> AGRLEEALELFEEMKEKGIVPDVVTYNTLISGLGKAGRLEEALELFEEMKEKGIVPDVVTYTTLISGLGKAGRLEEALELFEEMKEKGIVPNVVTYTTLISGLGKAGRLEEALELFEEMKEKGIVPDVVTYTTLISGLGKAGRLEEALELFEEMKEKGIVPDVVTYTTLISGLGKAGRLEEALELFEEMKEKGIVPDVVTYNTLISGLGKAGRLEEALELFEEMKEKGIVPDVVTYNTLISGLGKAGRLEEALELFEEMKEKGIVPDVVTYTTLISGLGKAGRLEEALELFEEMKEKGIVPNVVTYTTLISGLGKAGRLEEALELFEEMKEKGIVPDVVTYTTLISGLGK

PPR proteins are RNA-binding proteins found predominantly in mitochondria and chloroplasts. PPRs stack on each other to form an extended solenoid structure that can recognise RNA in a sequence-specific manner based on the identities of amino acids at positions 5 and 35 of each repeat. To bypass these limitations, we previously used consensus design to engineer artificial PPR domains (cPPRs) that are highly soluble and, via an appropriate choice of amino acids at position 5 and 35, can be designed to bind RNA in a predictable, sequence-specific manner. In this study we have discovered that cPPRs bind not only RNA but also ssDNA in a modular and programmable manner, analogous to their RNA-binding capability.

Next, we sought to obtain structural information on the two cPPR proteins specifically designed to bind to telomeric ssDNA sequences, to understand further the cPPR scaffold’s ability to bind both ssDNA and RNA. Although these proteins are highly similar in their primary sequences, only cPPR-Telo1 gave reproducible and diffracting crystals. We solved the structure of cPPR-Telo1 and cPPR-Telo1 bound to its ssDNA target using single-wavelength anomalous dispersion at 2.1 and 2.0 Å resolution, respectively (with sample electron densities in Supplementary Fig. 8). Mapping the electrostatic potential revealed a highly asymmetrical surface charge distribution with positively charged residues in the ssDNA-binding cavity and a negatively charged band along the exterior, exposed face of the superhelix. Our structures provide the first pair of structures where an identical PPR protein compacts upon binding a nucleic acid in the canonical, sequence-specific mode, providing an opportunity to understand how the conformation of the protein changes upon ligand binding. cPPR-Telo1 wraps around the ssDNA upon binding, inducing a massive compaction of the superhelical structure and decreasing the length of the protein from 104 to 64 Å. Overall, the rearrangement is based on the a helices on the concave side of the protein moving into closer proximity as bonds are formed to the DNA with a concomitant separation of the b helices on the convex side. To allow the separation, an extensive hydrogen bond network between an arginine at position 16 and a glutamic acid at position 19 from one PPR repeat and a glutamic acid at position 18 from the preceding repeat in the apo protein rearranges at three out of nine possible positions leading to a more open arrangement when bound to DNA.> MGSDKIHHHHHHMEKKIVYFNKPGRENTEETLRLAVERA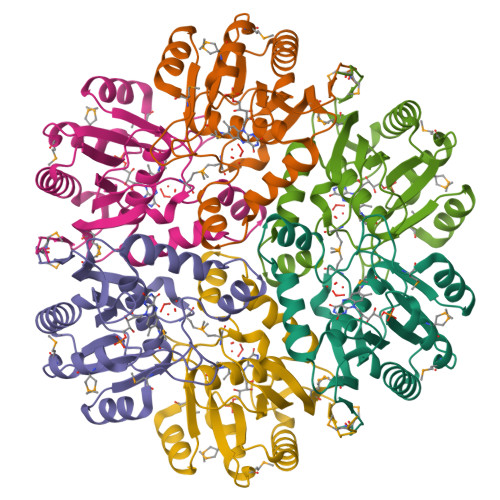KELGIKHLVVASSYGDTAMKALEMAEGLEVVVVTYHTGFVREGENTMPPEVEEELRKRGAKIVRQSHILSGLERSISRKLGGVSRTEAIAEALRSLFGHGLKVCVEITIMAADSGAIPIEEVVAVGGRSRGADTAVVIRPAHMNNFFDAEIKEIICMPRNKR>[4x]AASAQDAPEAETQAQETQGQAAARAAAADLAAGQDDEPRIL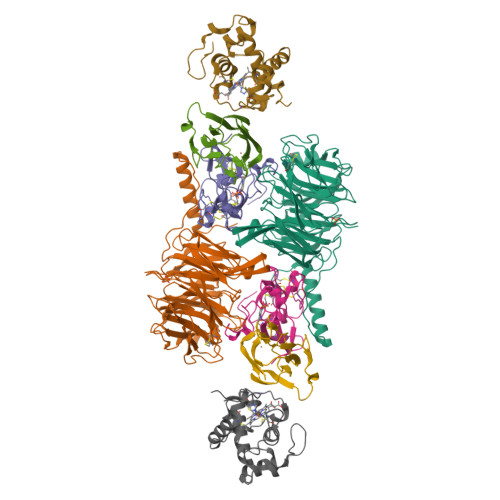EAPAPDARRVYVNDPAHAAAVTQQFVIDGEAGRVIGMIDGGFLPNPVVADDGSFIAHASTVFSRIARGERTDYVEVFDPVTLLPTADIELPDAPRFLVGTYPWMTSLTPDGKTLLFYQFSPAPAVGVVDLEGKAFKRMLDVPDCYHIFPTAPDTFFMHCRDGSLAKVAFGTEGTPEITHTEVFHPEDEFLINHPAYSQKAGRLVWPTYTGKIHQIDLSSGDAKFLPAVEALTEAERADGWRPGGWQQVAYHRALDRIYLLVDQRDEWRHKTASRFVVVLDAKTGERLAKFEMGHEIDSINVSQDEKPLLYALSTGDKTLYIHDAESGEELRSVNQLGHGPQVITTADMG;>[4x]ADAPAGTDPRAKWVPQDNDIQACDYWRHCSIDGNICDCSGGSLTNCPPGTKLATASWVASCYNPTDGQSYLIAYRDCCGYNVSGRCPCLNTEGELPVYRPEFANDIIWCFGAEDDAMTYHCTISPIVGKAS;>DKATIPSESPFAAAEVADGAIVVDIAKMKYETPELHVKVGDTVTWINREAMPHNVHFVAGVLGEAALKGPMMKKEQAYSLTFTEAGTYDYHCTPHPFMRGKVVVE[4x];>APQFFNIIDGSPLNFDDAMEEGRDTEAVKHFLETGENVYNEDPEILPEAEELYAGMCSGCHGHYAEGKIGPGLNDAYWTYPGNETDVGLFSTLYGGATGQMGPMWGSLTLDEMLRTMAWVRHLYTGDPKDASWLTDEQKAGFTPFQPKSSGEDQS[4x]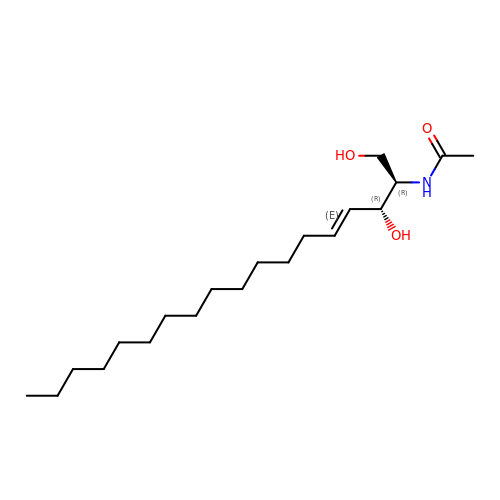N-[(1R,2R,3E)-2-hydroxy-1-(hydroxymethyl)heptadec-3-en-1-yl]acetamide | C20 H39 N O3 | BLTCBVOJNNKFKC-KTEGJIGUSA-N>QPALLRLSDHLLANYKKGVRPVRDWRKPTTVSIDVIMYAILNVDEKNQVLTTYIWYRQYWTDEFLQWTPEDFDNVTKLSIPTDSIWVPDILINEFVDVGKSPNIPYVYVHHRGEVQNYKPLQLVTACSLDIYNFPFDVQNCSLTFTSWLHTIQDINITLWRSPEEVRSDKSIFINQGEWELLEVFPQFKEFSIDISNSYAEMKFYVIIRRRPLFYAVSLLLPSIFLMVVDIVGFCLPPDSGERVSFKITLLLGYSVFLIIVSDTLPATAIGTPLIGVYFVVCMALLVISLAETIFIVRLVHKQDLQRPVPDWLRHLVLDRIAWILCLGEQPMAHRPPATFQANKTDDCSGSDLLPAMGNHCSHVGGPQDLEKTPRGRGSPLPPPREASLAVRGLLQ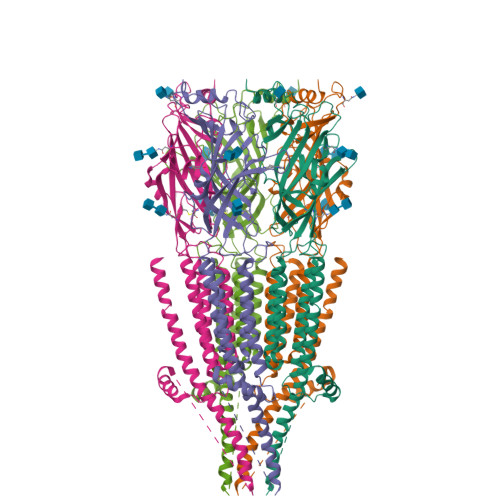ELSSIRHFLEKRDEMREVARDWLRVGYVLDRLLFRIYLLAVLAYSITLVTLWSIWH[5x]> SVNPHDMTSQQIVNDMKVGWNLG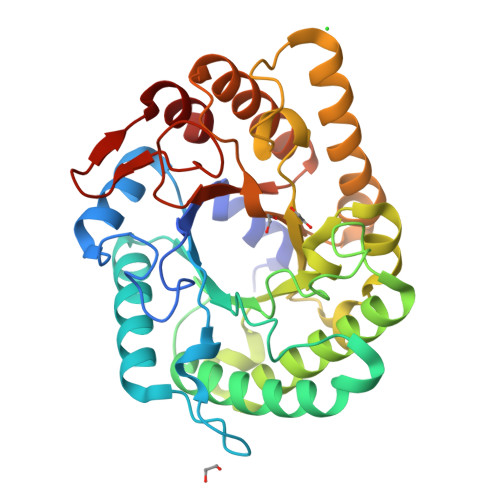NTLDASPDETGWGNPKTTKAMIDKIKEAGFNTVRIPVSWSSHIGAGPSYTIDQAWLNRVQEVVNYVIQDHMYAILNTHHDTSWIIPTYNKEAASTDELTKVWGQIANRFKDYDSHLIFQTLNEPRIVGSPEEWNGGTAESRDVINKFNLTAVNTIRSTGSNNSSRFIMVPTYAASTATAAMNDLVIPNNDKRVIVSLHMYAPYSFAMDPKGTSHWGGEADKDALDGQLNAIYNKFVKNGQPVVIGQFGSINKNNESSRASLAKFYVSDARKKGITTVWWDNGKSAVGDDNYGILDRNNLTWVFPKLVRTIVN>AELTVDQQTLLDYIMDSYSKQRMPQEITNKILKEEFSAEENFLILTEMATSHVQILVEFTKRLPGFQTLDHEDQIALLKGSAVEAMFLRSAEIFNKKLPAGHADLLEERIRKSGISDEYITPMFSFYKSVGELKMTQEEYALLTAIVILSPDRQYIKDREAVEKLQEPLLDVLQKLCKIYQPENPQHFACLLGRLTELRT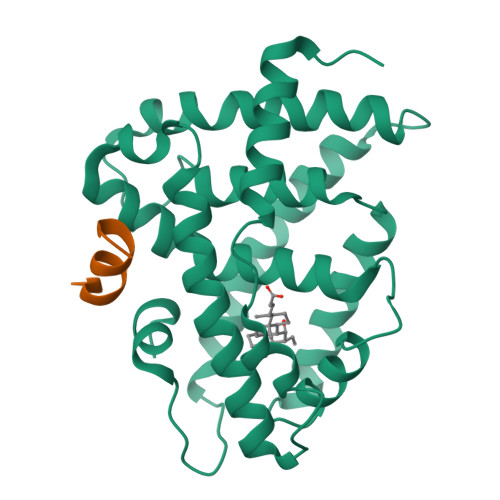FNHHHAEMLMSWRVNDHKFTPLLCEIWDVQ[2x];>ENALLRYLLDKD[3x]> 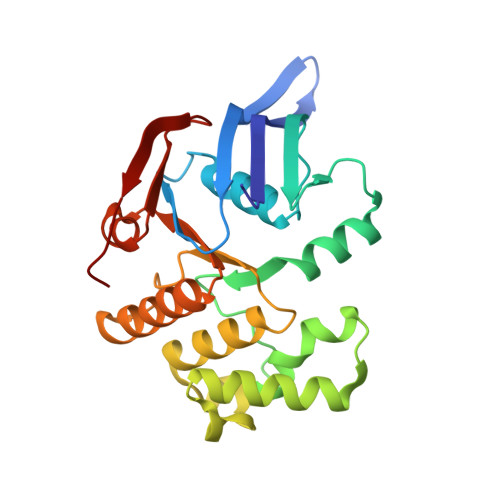MTPLLELKDIRRSYPAGDEQVEVLKGISLDIYAGEMVAIVGASGSGKSTLMNILGCLDKATSGTYRVAGQDVATLDADALAQLRREHFGFIFQRYHLLSHLTAEQNVEVPAVYAGLERKQRLLRAQELLQRLGLEDRTEYYPAQLSGGQQQRVSIARALMNGGQVILADEPTGALDSHSGEEVMAILHQLRDRGHTVIIVTHDPQVAAQAERVIEIRDGEIVRLEHHHHHH>DRWGSSLKPTAIESCMVKFELSSSKWHMTSPKPHCVNTTSDGKLKILQSGTYLIYGQVIPVDKKYIKDNAPFVVQIYKKNDVLQTLMNDFQILPIGGVYELHAGDNIYLKFNSKDHIQKNNTYWGIILMPDLPF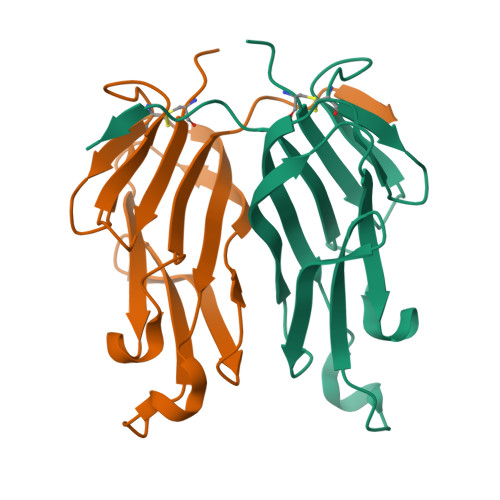IS[2x]>[2x]PHMPPLPPGWEEKVDNLGRTYYVNHNNRTTQWHRPSL;>EHRGPPPEYPFKGM[2x]

Several sets of host cell machinery facilitate this process, including proteins of the endosomal sorting complexes required for transport pathway, which mediates the membrane fission reaction required to complete viral budding, as well as angiomotin (AMOT) and NEDD4L, which bind one another and promote virion membrane envelopment. AMOT and NEDD4L interact through the four NEDD4L WW domains and three different AMOT Pro-Pro-x (any amino acid)-Tyr (PPxY) motifs, but these interactions are not yet well defined. Here, we report that individual AMOT PPxY and NEDD4L WW domains interact with the following general affinity hierarchies: AMOT PPxY1>PPxY2>PPxY3 and NEDD4L WW3>WW2>WW1∼WW4. Comparative structural, binding, and virological analyses reveal that complementary ionic and hydrophobic contacts on both sides of the WW–PPxY core interaction account for the unusually high affinity of the AMOT PPxY1–NEDD4L WW3 interaction.

To obtain structures, we screened a series of different high- and moderate-affinity AMOT PPxY–NEDD4L WW complexes for crystallization. Two such complexes, AMOT PPxY2–NEDD4L WW1 and AMOT PPxY2–NEDD4L WW2, yielded high-resolution crystal structures (1.52 Å and 1.74 Å, respectively). All five of our new structures exhibit canonical WW domains, with three-stranded β-sheets and canonical positioning of the two eponymous Trp residues. In all three WW–PPxY complexes, the PPxY core elements bind in an extended polyproline II helical conformation across the concave WW sheet. Each conserved residue in the PPxY motif makes canonical binding interactions: the first Pro/Leu residue binds in the “XP-groove,” where it stacks against the second conserved WW Trp residue (Trp525 in WW3). The second PPxY Pro packs against a Tyr/Phe residue from the second β-strand (β2), and its carbonyl oxygen forms a hydrogen bond to the hydroxyl of a conserved Thr (in β3). The fourth Tyr residue of PPxY binds in the characteristic “Y-pocket”, forming a hydrogen bond with conserved His (in loop-II between β2 and β3). Thus, the core WW–PPxY interactions are very similar in every case and apparently do not explain why AMOT PPxY1 binds WW3 with unusually high affinity. In contrast, the PPxY2–WW1 and PPxY2–WW2 complexes make few favorable contacts outside the core.>MGNASSIVQTINVTGDGNVFKPSAETSSTAVPSLSLSPGMLNPGGVPWIAVGDETSVTSPGALRRMTSKDIPETAIINTDNSSGAVPSESALVPYIDEPLVVVTEHAITNFTKAEMALEFNREFLDKMRVLSVSPKYSDLLTYVDCYVGVSARQALNNFQKQVPVITPTRQTMYVDSIQAALKALEKWEIDLRVAQTLLPTNVPIGEVSCPMQSVVKLLDDQLPDDSLIRRYPKEAAVALAKRNGGIQWMDVSEGTVMNEAVNAVAASALAPSASAPPLEEKSKLTEQAMDLVTAAEPEIIASLAPVPAPVFAIPPKPADYNVRTLRIDEATWLRMIPKSMNTPFQIQVTDNTGTNWHLNLRGGTRVVNLDQIAPMRFVLDLGGKSYKETSWDPNGKKVGFIVFQSKIPFELWTAASQIGQATVVNYVQLYAEDSSFTAQSIIATTSLAYNYEPEQLNKTDPEMNYYLLATFIDSAAITPTNMTQPDVWDALLTMSPLSAGEVTVKGAVVSEVVPADLIGSYTPESLNASLPNDAARCMIDRASKIAEAIKIDDDAGPDEYSPNSVPIQGQLAISQLETGYGVRIFNPKGILSKIASRAMQAFIGDPSTIITQAAPVLSDKNNWIALAQGVKTSLRTKSLSAGVKTAVSKLSSSESIQNWTQGFLDKVSAHFPAPKPDCPTSGDSGESSNRRVKRDSYAGVVKRGYTR[6x];>[3x]MEVCLPNGHQVVDLINNAFEGRVSIYSAQEGWDKTISAQPDMMVCGGAVVCMHCLGVVGSLQRKLKHLPHHRCNQQIRHQDYVDVQFADRVTAHWKRGMLSFVAQMHEMMNDVSPDDLDRVRTEGGSLVELNWLQVDPNSMFRSIHSSWTDPLQVVDDLDTKLDQYWTALNLMIDSSDLIPNFMMRDPSHAFNGVKLGGDARQTQFSRTFDSRSSLEWGVMVYDYSELEHDPSKGRAYRKELVTPARDFGHFGLSHYSRATTPILGKMPAVFSGMLTGNCKMYPFIKGTAKLKTVRKLVEAVNHAWGVEKIRYALGPGGMTGWYNRTMQQAPIVLTPAALTMFPDTIKFGDLNYPVMIGDPMILG;> MANVWGVRLADSLSSPTIETRTRQYTLHDLCSDLDANPGREPWKPLRNQRTNNIVAVQLFRPLQGLVLDTQLYGFPGAFDDWERFMREKLRVLKYEVLRIYPISNYSNEHVNVFVANALVGAFLSNQAFYDLLPLLIINDTMIGDLLGTGASLSQFFQSHGDVLEVAAGRKYLQMENYSNDDDDPPLFAKDLSDYAKAFYSDTYEVLDRFFWTHDSSAGVLVHYDKPTNGHHYLLGTLTQMVSAPPYIINATDAMLLESCLEQFSANVRARPAQPVTRLDQCYHLRWGAQYVGEDSLTYRLGVLSLLATNGYQLARPIPRQLTNRWLSSFVSQIMSDGVNETPLWPQERYVQIAYDSPSVVDGATQYGYVRKNQLRLGMRISALQSLSDTPSPVQWLPQYTIDQAAMDEGDLMVSRLTQLPLRPDYGNIWVGDALSYYVDYNRSHRVVLSSELPQLPDTYFDGDEQYGRSLFSLARKIGDRSLVKDTAVLKHAYQAIDPNTGKEYLRSRQSVAYFGASAGHSGADQPLVIEPWIQGKISGVPPPSSVRQFGYDVARGAIVDLARPFPSGDYQFVYSDVDQVVDGHDDLSISSGLVESLLSSCMHATAPGGSFVVKINFPTRPVWHYIEQKILPNITSYMLIKPFVTNNVELFFVAFGVHQHSSLTWTSGVYFFLVDHFYRYETLSTISRQLPSFGYVDDGSSVTGIETISIENPGFSNMTQAARIGISGLCANVGNARKSIAIYESHGARVLTITSRRSPASARRKSRLRYLPLIDPRSLEVQARTILPADPVLFENVSGASPHVCLTMMYNFEVSSAVYDGDVVLDLGTGPEAKILELIPATSPVTCVDIRPTAQPSGCWNVRTTFLELDYLSDGWITGVRGDIVTCMLSLGAAAAGKSMTFDAAFQQLIKVLSKSTANVVLVQVNCPTDVVRSIKGYLEIDSTNKRYRFPKFGRDEPYSDMDALEKICRTAWPNCSITWVPLSYDLRWTRLALLESTTLSSASIRIAELMYKYMPIMRIDIHGLPMEKRGNFIVGQNCSLVIPGFNAQDVFNCYFNSALAFSTEDVNAAMIPQVSAQFDATKGEWTLDMVFSDAGIYTMQALVGSNANPVSLGSFVVDSPDVDITDAWPAQLDFTIAGTDVDITVNPYYRLMTFVRIDGQWQIANPDKFQ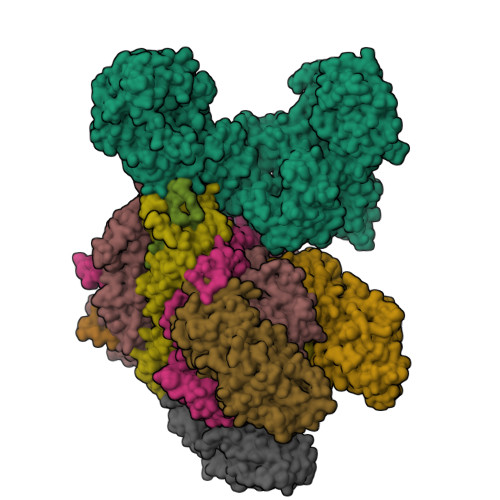FFSSASGTLVMNVKLDIADKYLLYYIRDVQSRDVGFYIQHPLQLLNTITLPTNEDLFLSAPDMREWAVKESGNTICILNSQGFVLPQDWDVLTDTISWSPSIPTYIVPPGDYTLTPL Dihydrofolate reductase (DHFR) is a key and essential enzyme in the folate pathway that converts dihydrofolate (DHF) to tetrahydrofolate (THF) (Raimondi et al., 2019). This coenzyme is required for a variety of cellular processes, including the synthesis of purine involved in nucleic acid and amino-acid biosynthesis. The active site is located in a cleft formed by α-helix 1, α-helix 2, α-helix 4 and β-sheet 1, similar to CglDHFR and CalDHFR. As classified in E. coli DHFR, CauDHFR could also be designated to have two subdomains: the nucleotide subdomain, in which the NADPH sits, and the substrate-binding subdomain, which is predominantly formed by α-helix 1, α-helix 2 and β-sheet 1.

The structure of apo CauDHFR was determined by molecular replacement using the structure of CalDHFR as a model, while the structures of the CauDHFR–NADPH, CauDHFR–NADPH–PYR and CauDHFR–NADPH–CYG complexes were also solved by molecular replacement using the structure of apo CauDHFR as a model. Crystals of apo and holo CauDHFR have a single protomer in the asymmetric unit, while the ternary complexes CauDHFR–NADPH–PYR and CauDHFR–NADPH–CYG contained two protein molecules which are independent and do not form a quaternary structure, according to the PISA server. Analysis of the NADPH binding sites of the four obtained structures shows that the holoenzyme and the CauDHFR–NADPH–PYR and CauDHFR–NADPH–CYG ternary complexes have the side chains of the NADPH binding site residues in similar conformations, whereas the apoenzyme has more significant differences. This could be caused by the conformational freedom imposed by the lack of cofactor. The substrate-binding regions of apo and holo CauDHFR are largely similar, with the addition of NADPH not making a substantial difference to most residue orientations. The main difference observed is movement of Leu25, with a change of 5 Å between the isopropyl functional groups. Minor movements are also seen in Met33, Thr57, Leu60 and Phe65.

> MSTRPKISLIVAALQPSMGIGAKGSLPWRLKNEMKYFKDVTSKAKDGHINAVVMGRKTWELIPERFRPLAGRLNVILSRKNDDLIDSNGVYHFSSFDSVMKHLEKDSFRFKDMPLDKIFIIGGSQIYNLLILDSRVDNLLVTQVHFVGEDADKPQMDTFLDWDLSKWKRLEHDKLEQYVGLDVPRGLNEEGSYNYEYTMWEKAQ>MSYYHHHHHHLESTSLYKKAGLNNFNLHTPTRILFGKGAIAGLREQIPHDARVLITYGGGSVKKTGVLDQVLDALKGMDVLEFGGIE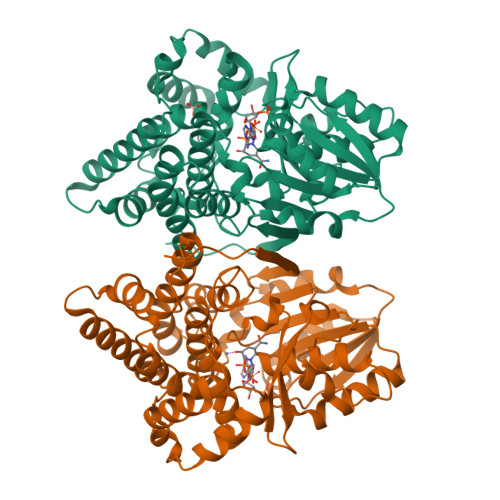PNPAYETLMNAVKLVREQKVTFLLAVGGGSVLDGTKFIAAAANYPENIDPWHILQTGGKEIKSAIPMGCVLTLPATGSESNAGAVISRKTTGDKQAFHSAHVQPVFAVLDPVYTYTLPPRQVANGVVDAFVHTVEQYVTKPVDAKIHDRFAEGILLTLIEDGPKALKEPENYDVRANVMWAATQALNGLIGAGVPQDWATHMLGHELTAMHGLDHAQTLAIVLPALWNEKRDTKRAKLLQYAERVWNITEGSDDERIDAAIAATRNFFEQLGVPTHLSDYGLDGSSIPALLKKLEEHGMTQLGENHDITLDVSRRIYEAAR[4x]> HHHHHHMSRLSEPSPYVEFDRRQWRALRMSTPLALTEEELVGLRGLGEQIDLLEVEEVYLPLARLIHLQVAARQRLFAATAEFLGEPQQNPDRPVPFIIGVAGSVAVGKSTTARVLQALLARWDHHPRVDLVTTDGFLYPNAELQRRNLMHRKGFPESYNRRALMRFVTSVKSGSDYACAPVYSHLHYDIIPGAEQVVRHPDILILEGLNVLQTGPTLMVSDLFDFSLY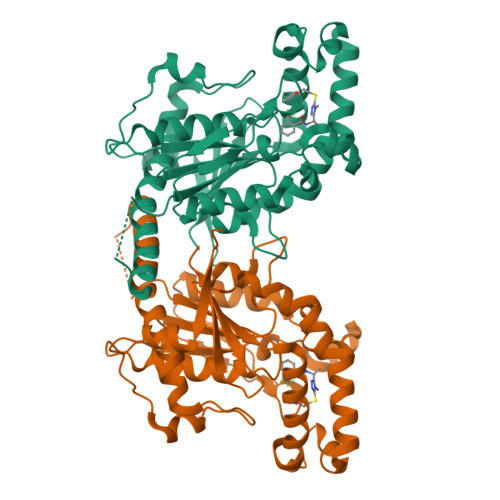VDARIEDIEQWYVSRFLAMRTTAFADPESHFHHYAAFSDSQAVVAAREIWRTINRPNLVENILPTRPRATLVLRKDADHSINRLRLRKL> SGHHDETTDEPSESSKPCCDQCSCTKSMPPKCRCSDIRLNSCHSACKSCACTYSIP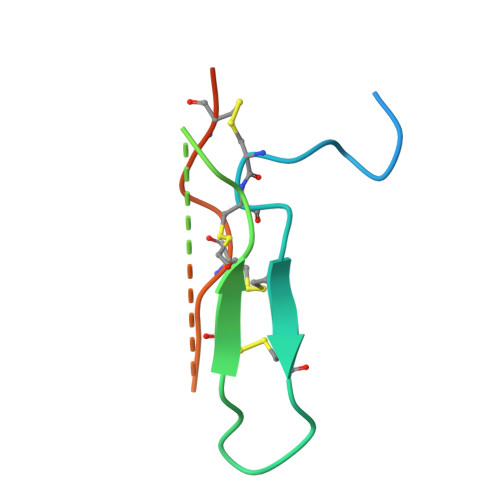AKCFCTDINDFCYEPCKSSRDDDWDN>[5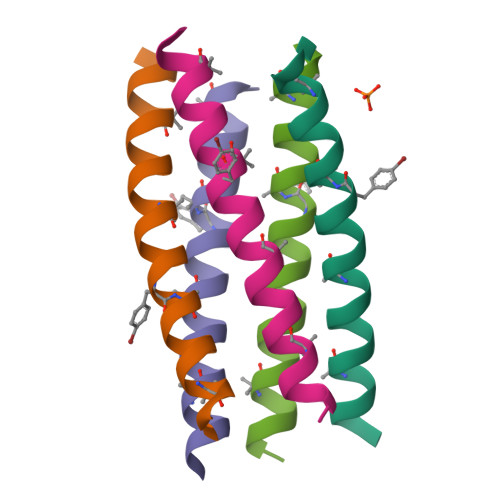x]XGEIAQALKEIAKALKEIAYALKEIAQALKGX> GPGSMAGAIASRMSFSSLKRKQPKTFTVRIVTMDAEMEFNCEMKWKGKDLFDLVCRTLGLRETWFFGLQYTIKDTVAWLKMDKKVLDHDVSKEEPVTFHFLAKFYPENAEEELVQEITQHLFFLQVKKQILDEKVYCPPEASVLLASYAVQAKYGDYDPSVHKRGFLAQEELLPKRVINLYQMTPEMWEERITAWYAEHRGRARDEAEMEYLKIAQDLEMYGVNYFTIRNKKGTELLLGVDALGLHIYDPENRLTPKISFPWNEIRNISYSDKEFTIKPLDKKIDVFKFNSSKLRVNKLILQLCIGNHDLFMRRRKAD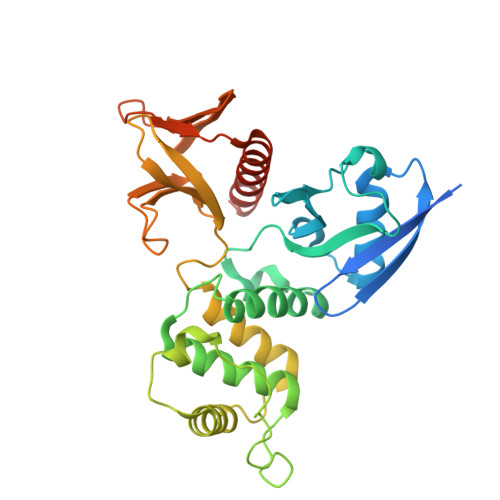SLEVQQ>[2x]MAKPANKLVIVTEKILLKKIAKIIDE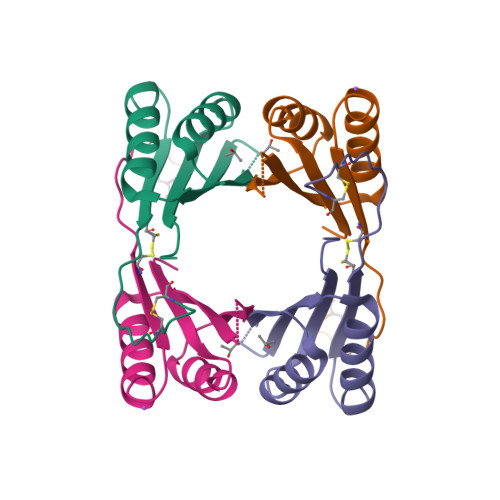SGAKGYTVMNTGGKGSRNVRSSGQPNTSDIEANIKFEILTETREMAEEIADRVAVKYFNDYAGIIYICSAEVLYGHTFCGPEGC>[2x]MVLYFIGLGLYDERDITVKGLEIAKKCDYVFAEFYTSLMAGTTLGRIQKLIGKEIRVLSREDVELNFENIVLPLAKENDVAFLTPGDPLVATTHAELRIRAKRAGVESYVIHAPSIYSAVGITGLHIYKFGKSATVAYPEGNWFPTSYYDVIKENAERGLHTLLFLDIKAEKAMYMTANEAMELLLKVEDMKKGGVFTDDTLVVVLARAGSLNPTI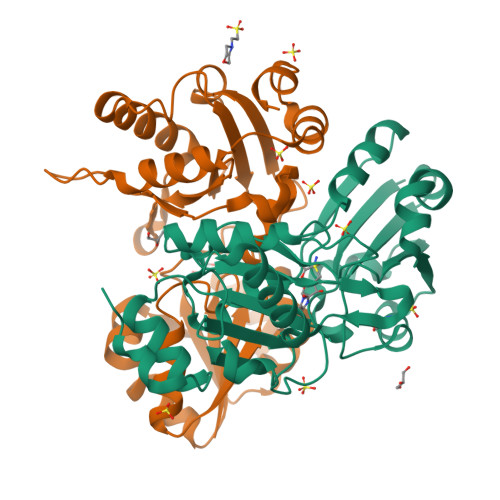RAGYVKDLIREDFGDPPHILIVPGKLHIVEAEYLVEIAGAPREILRVNV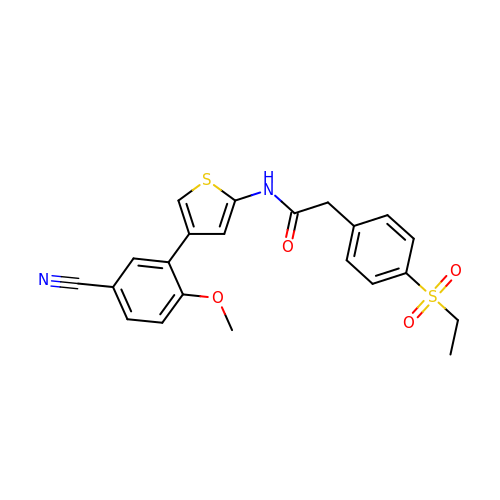~{N}-[4-(5-cyano-2-methoxy-phenyl)thiophen-2-yl]-2-(4-ethylsulfonylphenyl)ethanamide | C22 H20 N2 O4 S2 | QMPAKLUOYZNDSW-UHFFFAOYSA-N>MRVMITDKLRRDSEQIWKKIFEHPFVVQLYSGTLPLEKFKFYVLQDFNYLVGLTRALAVISSKAEYPLMAELIELARDEVTVEVENYVKLLKELDLTLEDAIKTEPTLVNSAYMDFMLATAYKGNIIEGLTALLPCFWSYAEIAEYHKDKLRDNPIKIYREWGKVYLSNEYLNLVGRLRKIIDSSGHSGYD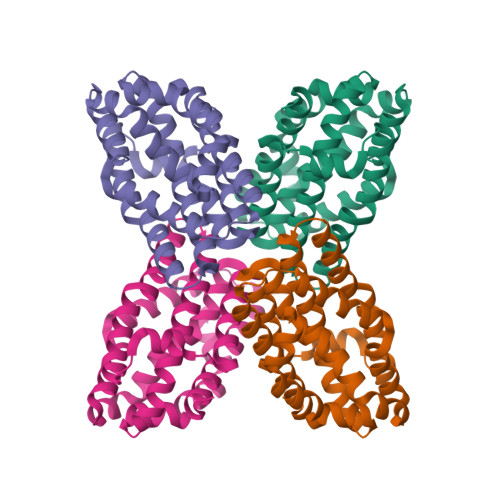RLRRIFITGSKFELAFWEMAWRGGDVFLEHHHHHH[4x]[3,5-bis(methylsulfanyl)-1,2-thiazol-4-yl]methanol | C6 H9 N O S3 | 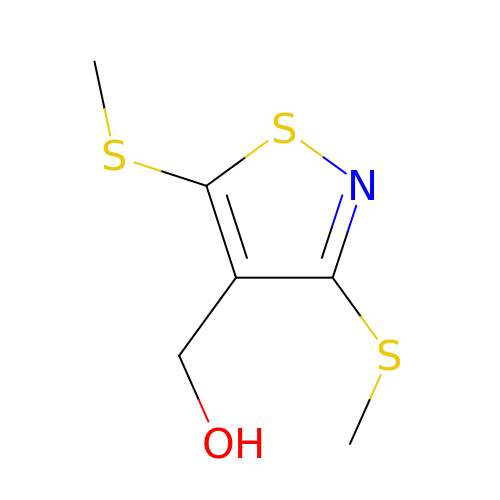SIFVTEYXNRZCMI-UHFFFAOYSA-N> MGRKKIQITRIMDERNRQVTFTKRKFGLMKKAY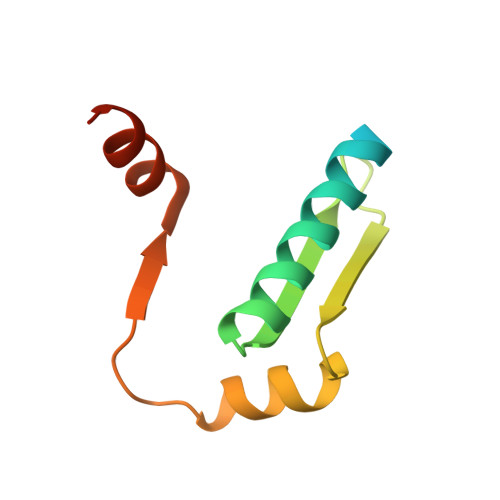ELSVLCDCEIALIIFNSTNKLFQYASTDMDKVLLKYTEYNEPHESRTNSDIVEALNKKENKG>MTTVVSRTFRSSPHRDALQTWDAIVELLTQGKDGTARSELRAVTGVAASLIADQAPKSAPIVATCDGPRTRIYCLFDEDAIDGDDANEEVLGFEPLKGDWGMSLPCPKEQLGWVQSALKKHSSRIIARDLSQGIATQAQADAGQAMSL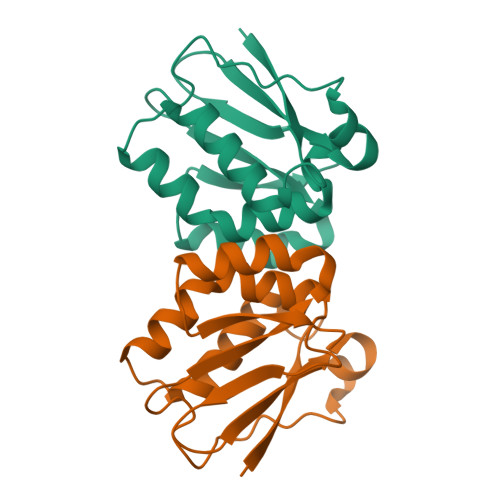DLGGFLKS[4x]>SNAMNYFDS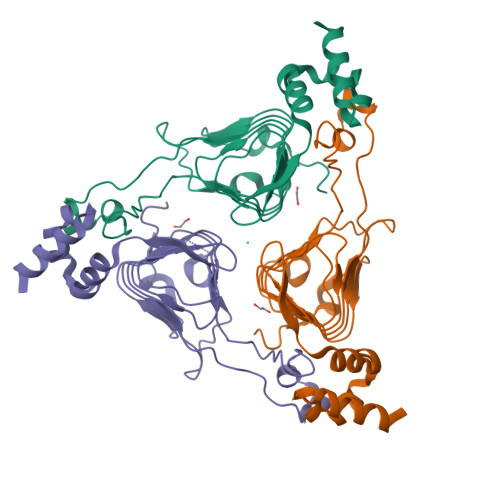PFSGKPIQEQITNPNIIVGRHSYYSGYYHGHGFDDCVRYLNPERNDVDKLIIGSFCSVGSGAVFMMAGNQGHRTDWVSTFPFFYQQNPNFSEAKDGFVRAGDTRIGHDVWIGSEAMIMPGVTIGDGAIIASRAVVTKDVAPYEVVGSNPAKHIKFRFSPQEIEMLQEMQWWQWSDEQLGQCMALMCSADIEGLYLWWKQSQ[3x]D-HISTIDINE | C6 H10 N3 O2 | 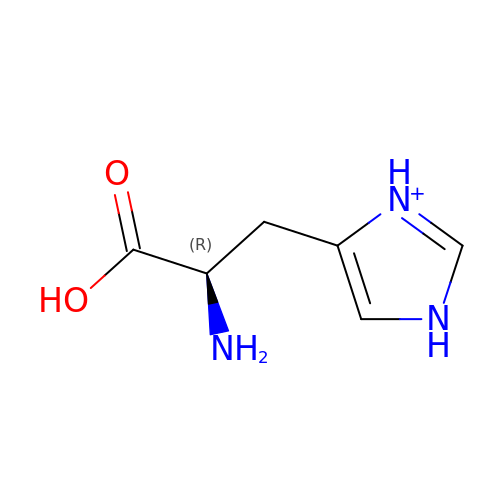HNDVDQJCIGZPNO-RXMQYKEDSA-O>GNSATSADEQPHIGNYRLLKTIGKGNFAKVKLARHILTGKEVAVRIIDKTQLNSSSLQKLFREVRIMKVLNHPNIVKLFEVIETEKTLYLVMEYASGGEVFDYLVAHGRMKEKEARAKFRQIVSAVQYCHQKFIVHRDLKAENLLLD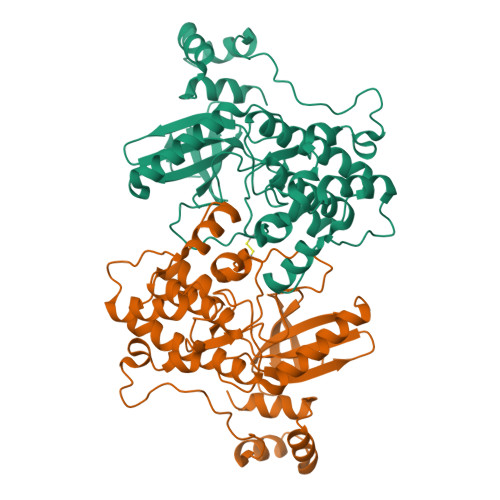ADMNIKIADFGFSNEFTFGNKLDEFCGSPPYAAPELFQGKKYDGPEVDVWSLGVILYTLVSGSLPFDGQNLKELRERVLRGKYRIPFYMSTDCENLLKKFLILNPSKRGTLEQIMKDRWMNVGHEDDELKPYVEPLPDYKDPRRTELMVSMGYTREEIQDSLVGQRYNEVMATYLLLGYK[6x]>MNGQGSDPAVTYYRLEEVAKHNTSESTWMVLHGRVYDLTRFLSEHPGGEEVLREQAGADATESFEDVGHSPDAR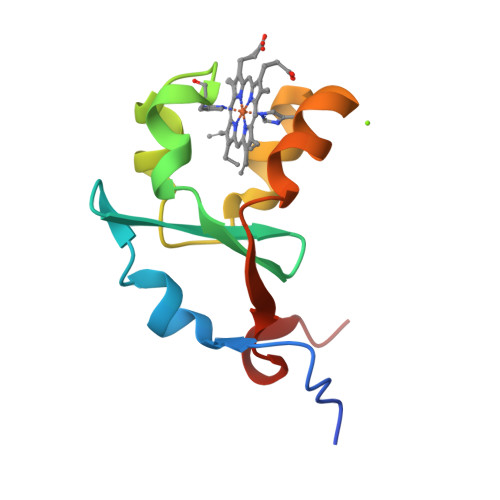EMSKQYYIGDVHPNDLKPK[4x]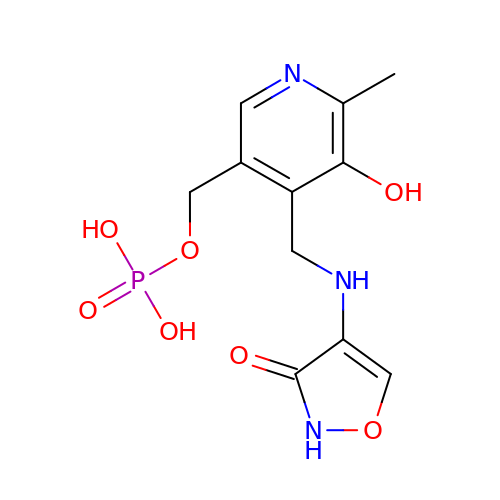(5-hydroxy-6-methyl-4-{[(3-oxo-2,3-dihydro-1,2-oxazol-4-yl)amino]methyl}pyridin-3-yl)methyl dihydrogen phosphate | C11 H14 N3 O7 P | PXWFNGNWQUPGPJ-UHFFFAOYSA-N> MLSQTSIPEVKEDVIGYALHQRRARVGQFQDLGPPDLITLIKSLPSSSSTTTATASANDNGATSNINGQDPTTIVTELHSHDKLKGQIGTFFYCMGIDTSDPTSITIFAKKITDLFLDTPQIWFGKKKHFHVSKISISSWNAFRKYDVNIIVHIPGTVQTYIINSDGEQSQLPSVAEASSGRNSQDLNVNMIWAETFMSGIVRDIMIMKDNRADGESQNLVETLIFNPFTSGELEDVANNFIKLFPLVYEKGVYLDAPTHVLNPSLTNNYLVETLVEIVRLTKSLEACRKMLKKLIEIHPEAVIILIRVYFACDLEIDAVDLINEQLNSPSSFLADDSKTSHIQLIFKSELLSIQSEFLLDVKRDYKLAKEVAMEAVNCAPNEFKTWYLL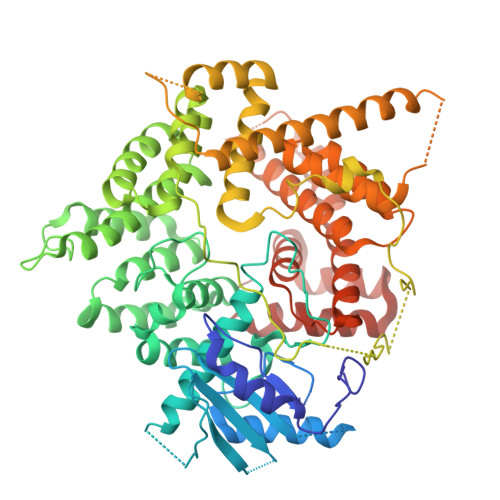TRIYIKLNDMSNALLSLNACPMSQVKEKYVLRRIAPITSDENLHLPLPLDASIEEISSLNPMDVQLEQKSADPNLVNLSASSLKSTFQLAYKLLTEIVQITGWEQLLKYRSKIFVMEDEYQGSTSSIDEAEVRGNDISKMRSKRLCERWLDNLFMLLYEDLKTYTDWQSEQLYFDAQNSKYHKLTVEWELFGLCAKRLGHLPEAAKAFQIGLSQRFSPVCAKNLLQFYIDEHKRIRRDSVSANSELTSSQILSSINDIDSSIIDLVVKICCWNHRWYIEFSIILIDALSVAVQDMGITKVHNEIASRFSDPVAQLIDDNILNFLKNFTNDTFDNGTENLYFQGHHHHHH>GDYYDYLFKIVLIGDSGVGKSNLLSRFTRDEFNLESKSTIGVEFATKSIQLKNNKIIKAQIWDTAGQERYRAITSAYYRGAVGALLVYDITKKNSFENIEKWLKELRDNADSNIVILLVGNKSDLKHLRVINDN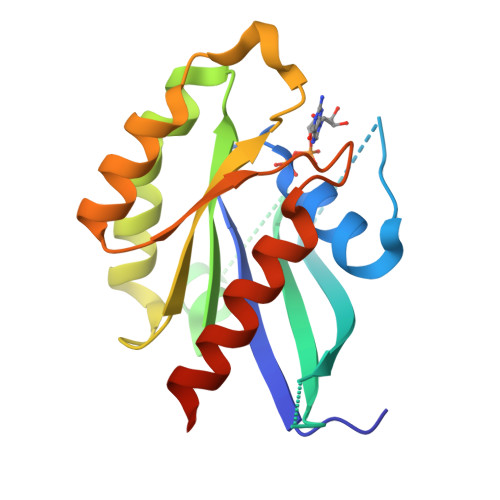DATQYAKKEKLAFIETSALEATNVELAFHQLLNEIYNVRQKKQATKN[5x]The AAA+ protein ClpC and the peptidase ClpP form a major bacterial proteasome with crucial functions in bacterial stress resistance and virulence. ClpC forms a hexameric ring and threads substrates under ATP consumption through its central channel into the proteolytic chamber of associated ClpP for degradation. ClpC is usually repressed in an inactive resting state, where two ClpC spirals interact via coiled-coil M-domains. Antibacterial peptides and partner proteins trigger ClpC activation by binding to its N-terminal domain (NTD). This study reveals that the NTD stabilizes the resting state through multiple anchoring points to M-domains and ATPase domains.

ClpC-WT formed three distinct species in presence of ATP that corresponded to complexes consisting of 10, 12 and 14 subunits. This finding was important in informing the cryo-EM data analysis and guiding us to classify and refine three distinct maps corresponding to the 10-, 12- and 14-mer at a resolution of around 3.8 Å (Movie EV1). The three oligomeric states aligned to each other almost perfectly (CC of 0.89) on the “front side” of the double staircase while they differ in the “back side”, which is open as a cradle in the 10-mer and closed with a seam in the 14-mer. Upon signal subtraction and local refinement of dimers from the 14-mer dataset, we obtained the highest-resolution map (3.5 Å) of a ClpC resting-state dimer (see “Methods”) then merged into a 14-mer combined map. The increased resolution of the 14-mer resting state and the generation of an improved AlphaFold2 model of the S. aureus ClpC monomer allowed us to partially refine the full resting state structure and to precisely position the NTD into the cryo-EM density. Out of the 14 ATP-binding sites at AAA2, 8 are occupied with nucleotides (7 ATPs and 1 ADP). While loaded, the ATPase activity of AAA2 will remain low as the highly-pitched assembly of the ATP pockets prevents allosteric arginine-fingers (R704) from neighboring subunits to access bound nucleotides (average distance 9 Å) and trigger ATP hydrolysis. Seam subunits NTDs of the 14-mer state make contact with different domains in the inner surface of the assembly (Movie EV2). In particular, NTD residue K85 makes intra-subunit salt bridge interactions with residues D356 and E359 of the AAA1, highlighting a possible regulatory contact that connects the ATPase domain with the NTD. Each NTD also makes extensive contacts with the MD of the adjacent subunit (MD*), mainly mediated by a patch of hydrophobic and apolar amino acids and one clear salt bridge between conserved residues R9 and E435.

>[14x]MLFGRLTERAQRVLAHAQEEAIRLNHSNIGTEHLLLGLMKEPEGIAAKVLESFNITEDKVIEEVEKLIGHGQDHVGTLHYTPRAKKVIELSMDEARKLHHNFVGTEHILLGLIRENEGVAARVFANLDLNITKARAQVVKALGNPEMSNKNAQASKSNNTPTLDSLARDLTVIAKDGTLDPVIGRDKEITRVIEVLSRRTKNNPVLIGEPGVGKTAIAEGLAQAIVNNEVPETLKDKRVMSLDMGTVVAGTKYRGEFEERLKKVMEEIQQAGNVILFIDELHTLVGAGGAEGAIDASNILKPALARGELQCIGATTLDEYRKNIEKDAALERRFQPVQVDEPSVVDTVAILKGLRDRYEAHHRINISDEAIEAAVKLSNRYVSDRFLPDKAIDLIDEASSKVRLKSHTTPNNLKEIEQEIEKVKNEKDAAVHAQEFENAANLRDKQTKLEKQYEEAKNEWKNAQNGMSTSLSEEDIAEVIAGWTGIPLTKINETESEKLLSLEDTLHERVIGQKDAVNSISKAVRRARAGLKDPKRPIGSFIFLGPTGVGKTELARALAESMFGDDDAMIRVDMSEFMEKHAVSRLVGAPPGYVGHDDGGQLTEKVRRKPYSVILFDEIEKAHPDVFNILLQVLDDGHLTDTKGRTVDFRNTIIIMTSNVGAQELQDQRFAGFGGSSDGQDYETIRKTMLKELKNSFRPEFLNRVDDIIVFHKLTKEELKEIVTMMVNKLTNRLSEQNINIIVTDKAKDKIAEEGYDPEYGARPLIRAIQKTIEDNLSELILDGNQIEGKKVTVDHDGKEFKYDIAEQTSETKTPSQA>[4x]ADCPPGWSSYDLYCYQGFNGPQTWDDAERFCTEQAKGGHLVSISDSGEADFVGQLITQNISRPEYYVWTGLRDRRSEQQCNPEWNDGSSIIYTNWDSGESEMCQAFSRWTNFREWMNTNCQQKNPFVCKFPPA;>DCPSGWSSYDGHCYQVFSDLKNWDDAESFCSGQHEGSRLASIHSREEEAFVGKMASRTLKYTSMWLGLNNPWKECKWEWSDDTRLDYKVWTRRPYCTVMVVKTDRIFW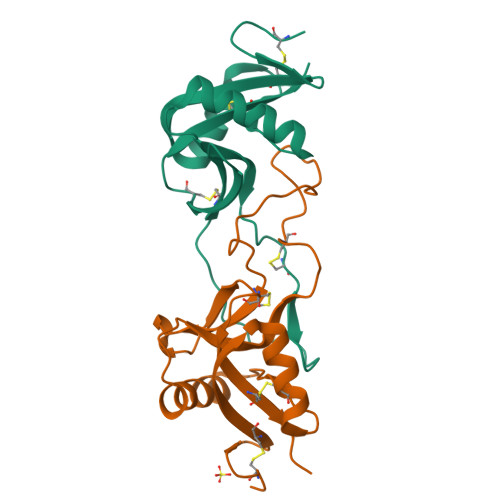FNRGCEKSVSFVCKFKAYSEDAAE[4x]>RAHKETLDKLTNAAINKINLLNTSKVKYLVSSAFAGLYVGIGILLIFTIGGLLTDAGSPMTKIVMGLSFAIALSLVIMTGTELFTGNNMVMSAGMLNKGVSIKDTSKIWAYSWVGNLIGALVLGIIFVGTGLVDKGPVAEFFANTAASKASMPFTALFFRGILCNILVCVSVLCSFRTNSDTAKIIMIFLCLFAFITSGFEHSVANMTIYSVSLFSPTISTVTIGGAIYNLVAVTLGNIVGGALFMGLGTY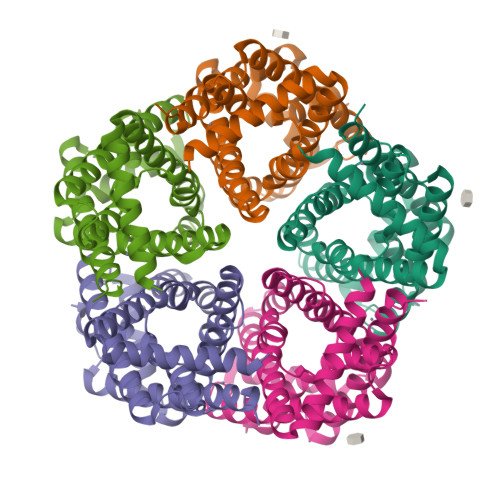ILGKEK[5x]Sortilin can trigger internalization of ligands from the cell surface via endocytosis and sorts ligands between several intracellular compartments, such as the trans-Golgi network (TGN), endosomes, lysosomes, and the secretory pathway. Sortilin binds and sorts a broad range of ligands, and dysfunction of sortilin has been linked to a wide range of disorders. Previously solved crystal structures of s-sortilin revealed that the Vps10p domain in fact consists of three domains; a ten-bladed β-propeller and two 10CC domains (10CC-a and 10CC-b) that have substantial interactions with the β-propeller. In this study, we detail that sortilin undergoes a conformational change within the three luminal domains and dimerizes while transitioning from neutral to acidic pH.

We determined the structures of the glycosylated luminal segment of mouse sortilin, s-sortilin, from crystals grown at neutral pH (pH 7.5, one crystal form, 2.1 Å maximum resolution) and acidic pH (pH ranging from 5.0 to 6.2, three crystal forms, maximum resolution ranging from 2.3 to 4.0 Å). The structures reveal two distinct conformations, a monomer at neutral pH and a dimer at acidic pH. The eight independent s-sortilin molecules in the three crystal forms grown at acidic pH all form homodimers with an identical interface and highly similar structure. The r.m.s.d. between the s-sortilin chains in the dimers is 0.80 Å for all of the 650 Cα atoms modeled. S-sortilin dimerizes through the top face of the β-propeller, i.e., the large side of the β-propeller disk opposite to the bottom face at which the 10CC domains are located. The predominantly hydrophobic dimer interface is large with a buried surface area of 4882 Å2 and is formed mainly by loops protruding from the blades. β-Propeller blades 1, 4, 6, 7, 8, 9, and 10 are involved in dimer formation. In the s-sortilin dimer the C-termini are in close proximity to each other with 37 Å distance between the two N713 Cα atoms. The s-sortilin dimer structures, crystallized at acidic pH, reveal that dimerization is accompanied by a substantial conformational rearrangement within the ß-propeller and two 10CC domains. Despite three internal disulfide bonds in 10CC-b, the three α-helices that form a small hydrophobic core in the s-sortilin monomer change their conformation into a three-stranded β-sheet in the dimer. In the monomer conformation, the s-sortilin C-terminus is exposed and pointing away from the β-propeller; whereas in the dimer conformation, it is interacting, through conserved hydrophobic interactions, with the rim of the β-propeller at blades 4 and 5.

>QDRLDAPPPPAPPLLRWAGPVGVSWGLRAAAPGGPVPRAGRWRRGAPAEDQDCGRLPDFIAKLTNNTHQHVFDDLSGSVSLSWVGDSTGVILVLTTFQVPLVIVSFGQSKLYRSEDYGKNFKDITNLINNTFIRTEFGMAIGPENSGKVILTAEVSGGSRGGRVFRSSDFAKNFVQTDLPFHPLTQMMYSPQNSDYLLALSTENGLWVSKNFGEKWEEIHKAVCLAKWGPNNIIFFTTHVNGSCKADLGALELWRTSDLGKTFKTIGVKIYSFGLGGRFLFASVMADKDTTRRIHVSTDQGDTWSMAQLPSVGQEQFYSILAANEDMVFMHVDEPGDTGFGTIFTSDDRGIVYSKSLDRHLYTTTGGETDFTNVTSLRGVYITSTLSEDNSIQSMITFDQGGRWEHLRKPENSKCDATAKNKNECSLHIHASYSISQKLNVPMAPLSEPNAVGIVIAHGSVGDAISVMVPDVYISDDGGYSWAKMLEGPHYYTILDSGGIIVAIEHSNRPINVIKFSTDEGQCWQSYVFTQEPIYFTGLASEPGARSMNISIWGFTESFITRQWVSYTVDFKDILERNCEEDDYTTWLAHSTDPGDYKDGCILGYKEQFLRLRKSSVCQNGRDYVVAKQPSVCPCSLEDFLCDFGYFRPENASECVEQPELKGHELEFCLYGKEEHLTTNGYRKIPGDKCQGGMNPAREVKDLKKKCTSNFLNPTKQNSKSNAAAHHHHHH[2x]> MAKLDKEQVIDNALILLNEVGIEGLTTRKLAQKIGVEQPT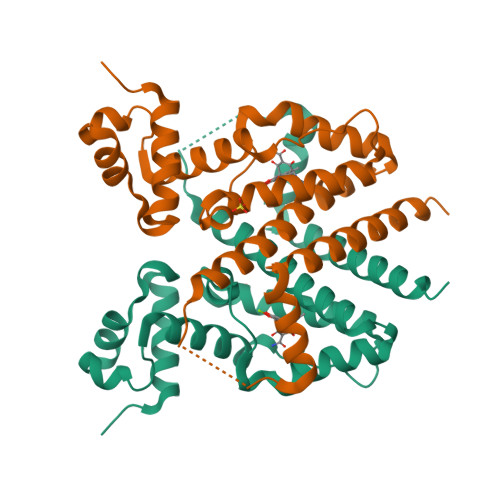LYWHVKNKRALLDALAETILQKHHHHVLPLPNETWQDFLRNNAKSFRQALLMYRDGGKIHAGTRPSESQFETSEQQLQFLCDAGFSLSQAVYALSSIAHFTLGSVLETQEHQESQKEREKVETDTVAYPPLLTQAVAIMDSDNGDAAFLFVLDVMISGLETVLKSAK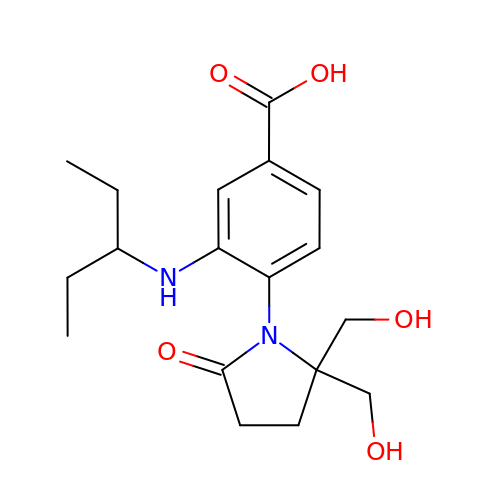1-[4-CARBOXY-2-(3-PENTYLAMINO)PHENYL]-5,5'-DI(HYDROXYMETHYL)PYRROLIDIN-2-ONE | C18 H26 N2 O5 | BNIJJJRESBVRNB-UHFFFAOYSA-N>GSHMDNSASKNSAISSSIFCEKYKQTKEQALTFFQEHPQYMRSKEDEEQLMTEFKKVLLEPGSKNLSI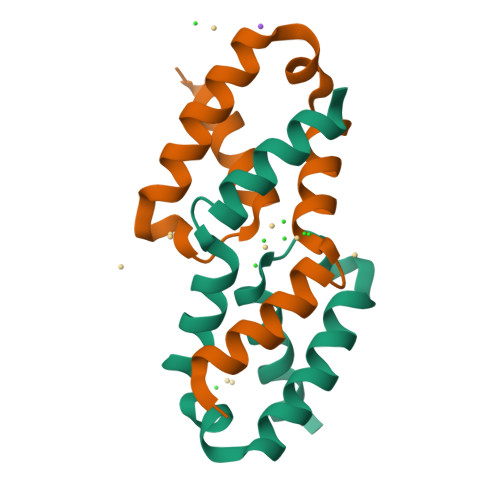YQTLLAAHERLQAL[4x]>MAQQSTKNETALLVAKSAKSALQDFNHDYSKSWTFGDKWDNSNTMFETFVNKYLFPKINETLLIDIALGNRFNWLAKEQDFIGQYSEEYVIMDTVPINMDLSKNEELMLKRNYPRMATKLYGNGIVKKQKFTLNNNDTRFNFQTLADATNYALGVYKKKISDINVLEEKEMRAMLVDYSLNQLSETNVRKATSKEDLASKVFEAILNLQNNSAKYNEVHRASGGAIGQYTTVSKLKDIVILTTDSLKSYLLDTKIANTFQIAGIDFTDHVISFDDLGGVFKVTKEFKLQNQDSIDFLRAYGDYQSQLGDTIPVGAVFTYDVSKLKEFTGNVEEIKPKSDLYAFILDINSIKYKRYTKGMLKPPFHNPEFDEVTHWIHY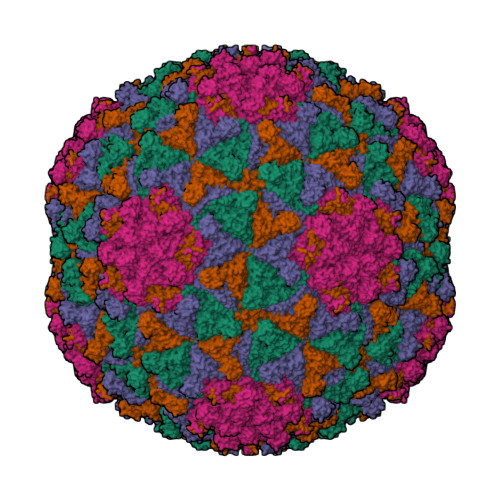YSFKAISPFFNKILITDQDVNPKPEEELQE[4x];>[4x]MYEGNNMRSMMGTSYEDSRLNKRTELNENMSIDTNKSEDSYGVQIHSLSKQSFTGDVEEE>[2x]GAELPAPLRRTGVGEWLATTCQGCTSWCAKQIYVMDGRALKVRGNPNSGVHGMSSCPRQHLSLQQVYDPDRLR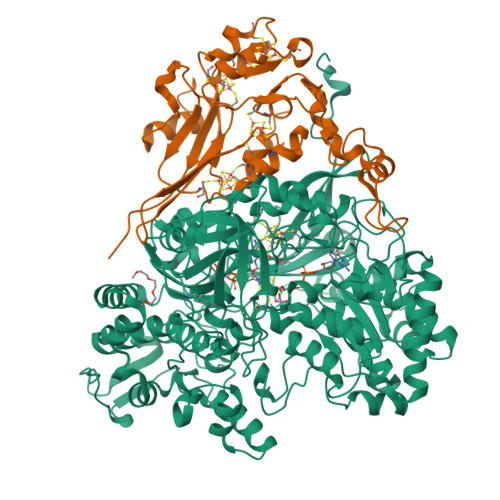TPMMRTNPKKGRDQDPKFVPISWDKALDMLADKIIALRVANEPHKYALLRGRYSHINDLLYKKMTNLIGSPNNISHSSVCAEAHKMGPYYLDGNWGYNQYDVKNAKFILSFGADPIASNRQVSFYSQTWGDSLDHAKVVVVDPRLSASAAKAHKWIPIEPGQDSVLALAIAHVALVEGVWHKPFVGDFIEGKNLFKAGKTVSVESFKETHTYGLVEWWNQALKDYTPEWASKITGIDPKTIIAIAKDMGAAAPAVQVWTSRGAVMQARGTYTSISCHALNGLFGGIDSKGGLFPGNKTPLLKEYPEAKAYMDEIAAKGVKKEKIDQRGRLEFPALAKGKSGGGVITANAANGIRNQDPYEIKVMLAYFNNFNFSNPEGQRWDEALSKVDFMAHITTNVSEFSWFADVLLPSSHHMFEKWGVLDSIGNGVAQISIQQPSIKRLWDTRIDESEIPYMLAKKLADKGFDAPWRYINEQIVDPETGKPAADEAEFAKLMVRYLTAPLWKEDASKYGDKLSSWDEFVQKGVWNSSPYKLEARWGKFKTETTKFEFYSKTLEKALQSHADKHKVSIDEVMKACDYQARGHLAFIPHYEEPYRFGDESEFPLLLVDQKSRLNKEGRTANSPWYYEFKDVDPGDVANEDVAKFNPIDGKKFGLKDGDEIRITSPVGMLTCKAKLWEGVRPGTVAKCFGQGHWAYGRYASAKFGVTPRGGSNNDLIADRYDRLSGASAFYGHIRVRVEKV;>MRLGMVIDLQKCVGCGGCSLACKTENNTNDGIHWSHHIATTEGTFPDVKYTYIPTLCNHCDDAPCVKVCPTGAMHKDKRGLTLQNNDECIGCKKCMNACPYGVISFNAATPHRRWQDDSEVVANGTVSPLMLLKRTGATATPNENPERGDTYPMIRPKRTTEKCTFCDHRLDKGLNPACVDACPSEARVIGDLDDPQSKVSQLIKLHKPMQLKPEAGTGPRVFYIRSFGVKTAY[2x]(1S)-6-chloro-2,3,4,9-tetrahydro-1H-carbazole-1- 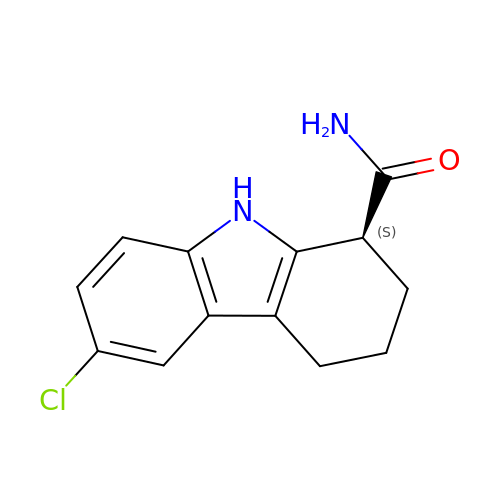carboxamide | C13 H13 Cl N2 O | FUZYTVDVLBBXDL-VIFPVBQESA-N>[2x]MGYSSDTTPCCFAY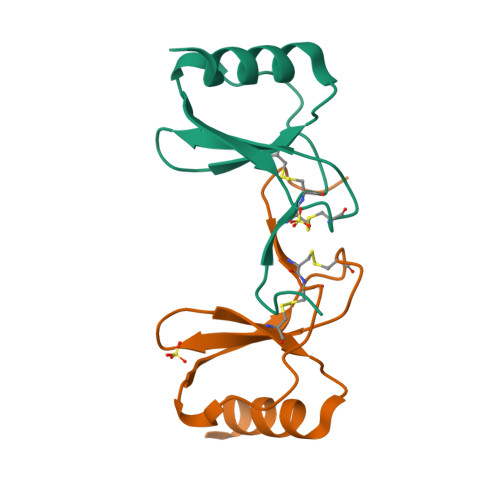IARPMPRAHIKEYFYTSGKCSNPAVVFVTRKNRQVCANPEKKWVREYINSLEMS>MNTYNPFRLDAPSMLLIEEWNQTAETGGQVTAGFTTKNGGESEPPFHSLNTGLHVQDHEQHVINNRKKVADILKTDLHDWVFADQTHEDRIHKVTDGDRASGAFRYDTALKATDGLYTDRPNLFLALCFADCVPVYFYDPVRSLVGIAHAGWKGTALGIAASMVDMWIRREGSNPADIRAVIGPAIGSCCYTVDDHVIDKIRNLPLQQEDKAFLTIKEGEYRLELKEVNRQLLVHA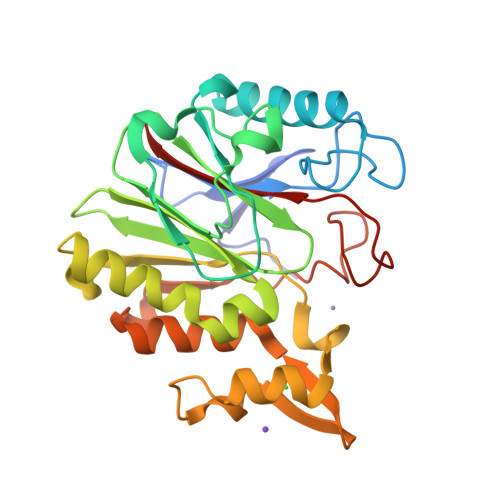GIPNGQIEVSSLCTSCERSLFFSHRRDRGKTGRMMSFIGLKEV[2x]> MESKEPQLKGIVTRLFSQQGYFLQMHPDGTIDGTKDENSDYTLFNLIPVGLRVVAIQGVKASLYVAMNGEGYLYSSD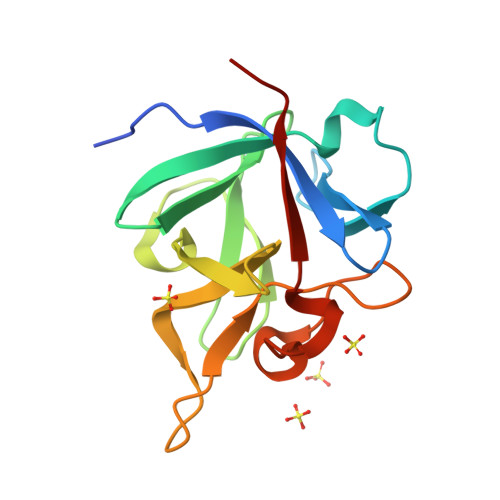VFTPECKFKESVFENYYVIYSSTLYRQQESGRAWFLGLNKEGQIMKGNRVKKTKPSSHFVPKPIEVA> KIRPECFELLRVLGKGGYGKVFQVRKVTGANTGKIFAMKVLKKAMIVRNAKDTAHTKAERNILEEVKHPFIVDLIYAFQTGGKLYLILEYLSGGELFMQLEREGIFMEDTACFYLAEISMAL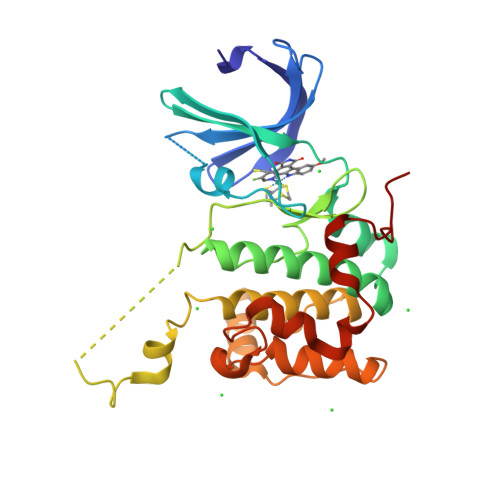GHLHQKGIIYRDLKPENIMLNHQGHVKLTDFGLCKESIHDGTVTHTFCGTIEYMAPEILMRSGHNRAVDWWSLGALMYDMLTGAPPFTGENRKKTIDKILKCKLNLPPYLTQEARDLLKKLLKRNAASRLGAGPGDAGEVQAHPFFRHINWEELLARKVEPPFKPL>[4x]SMTPYEDLLRFVLETGTPKSDRTGTGTRSLFGQQMRYDLSAGFPLLTTKKVHFKSVAYELLWFLRGDSNIGWLHEHGVTIWDEWASDTGELGPIYGVQWRSWPAPSGEHIDQISAALDLLRTDPDSRRIIVSAWNVGEIERMALPPCH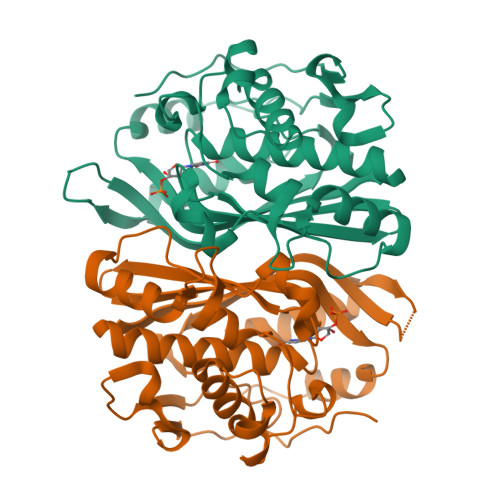AFFQFYVADGRLSCQLYQRSADLFLGVPFNIASYALLTHMMAAQAGLSVGEFIWTGGDCHIYDNHVEQVRLQLSREPRPYPKLLLADRDSIFEYTYEDIVVKNYDPHPAIKAPVAV> GAGCAACUUAGGAUUUUAGGCUCCCCGGCGUGUCUCGAACCAUGCCGGGCCGAACCCAUAGGGCUGGCGGUCCCUGUGCGGUC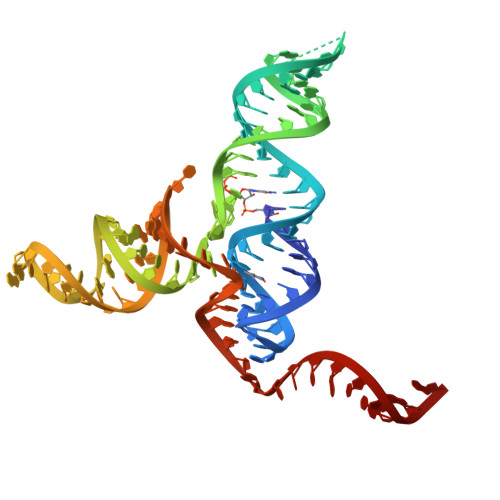AAAAUUCAUCCGCCGGAG> GSQEKAVVLDEQAIRRALT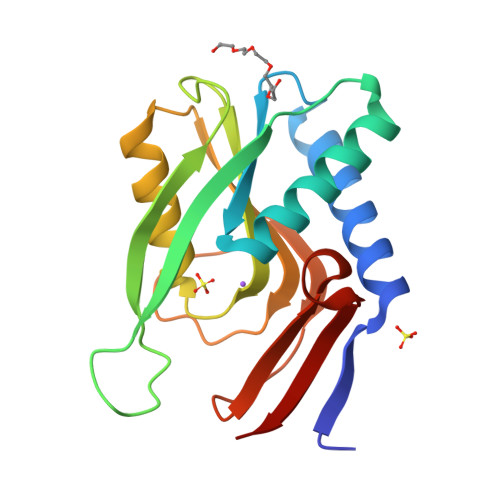RIAHEIIERNKGVDNCVLVGIKTRGIYLAKRLAERIEQIEGKPVPVGEIDITLYRDDLTVTSNKEPLVKGTDIPVDITDKKVILVDDVLYTGRTVRAGMDALMDLGRPSQIQLAVLVDRGHRELPIRADYVGKNVPTSKSERIVVQLSEVDGQDRVSIYEK>DALKVNRAPVGVEPQEVHKWLQSFNWDFKENRTKYPTKYHMANETKEQFKVIAKEYARMEAAKDERQFGTLLDGLTRLGAGNKVHPRWGETMKVISNFLEVGEYNAIAASAMLWDSATAAEQKNGYLAQVLDEIRHTHQCAFINHYYSKHYHDPAGHNDARRTRAIGPLWKGMKRVFADGFISGDAVECSVNLQLVGEACFTNPLIVAVTEWASANGDEITPTVFLSVETDELRHMANGYQTVVSIANDPASAKFLNTDLNNAFWTQQKYFTPVLGYLFEYGSKFKVEPWVKTWNRWVYEDWGGIWIGRLGKYGVESPASLRDAKRDAYWAHHDLALAAYAMWPLGFARLALPDEEDQAWFEANYPGWADHYGKIFNEWKKLGYEDPKSGFIPYQWLLANGHDVYIDRVSQVPFIPSLAKGTGSLRVHEFNGKKHSLTDDWGERQWLIEPERYECHNVFEQYEGRELSEVIAEGHGVRSDGKTLIAQPHTRGDNLWTLEDIKRAGCVFPDPLAKF[2x];>[2x]PQSSQVTKRGLTDPERAAIIAAAVPDHALDTQRKYHYFIQPRWKRLSEYEQLSCYAQPNPDWIAGGLDWGDWTQKFHGGRPSWGNESTELRTTDWYRHRDPARRWHHPYVKDKSEEARYTQRFLAAYSSEGSIRTIDPYWRDEILNKYFGALLYSEYGLFNAHSSVGRDCLSDTIRQTAVFAALDKVDNAQMIQMERLFIAKLVPGFDASTDVPKKIWTTDPIYSGARATVQEIWQGVQDWNEILWAGHAVYDATFGQFARREFFQRLATVYGDTLTPFFTAQSQTYFQTTRGAIDDLFVYCLANDSEFGAHNRTFLNAWTEHYLASSVAALKDFVGLYAKVEKVAGATDRAGVSEALQRVFGDWKIDYADKIGFRVDVDQKVDAVLAGYKN;>[2x]AKREPIHDNSIRTEWEAKIAKLTSVDQATKFIQDFRLAYTSPFRKSYDIDVDYQYIERKIEEKLSVLKTEKLPVADLITKATTGEDAAAVEATWIAKIKAAKSKYEAERIHIEFRQLYKPPVLPVNVFLRTDAALGTVLMEIRNTDYYGTPLEG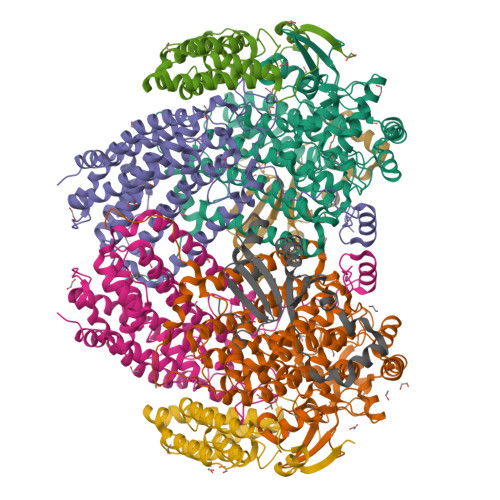LRKERGVKVLHLQA;>SAHNAYNAGIMQKTGKAFADEFFAEENQVVHESNAVVLVLMKSDEIDAIIEDIVLKGGKAKNPSIVVEDKAGFWWIKADGAIEIDAAEAGELLGKPFSVYDLLIGVSATVGRAYTLGTKFTITSELMGLDRALTDI[2x]> TCGLRKYKEPQLHSTGGLFTDITSHPWQAAIFAQNRRSSGERFLCGGILISSCWVLTAAHCFQESYLPDQLKVVLGRTYRVKPGEEEQTFKVKKYIVHKEFDDDTYNNDIALLQLKSDSPQCAQESDSVRAICLPEANLQLPDWTECELSGYGKHKSSSPFYSEQLKEGHVRLYPSSRCAPKFLFNKTVTNNMLCAGDTRSGEIYPNVHDACQGDSGGPLVCM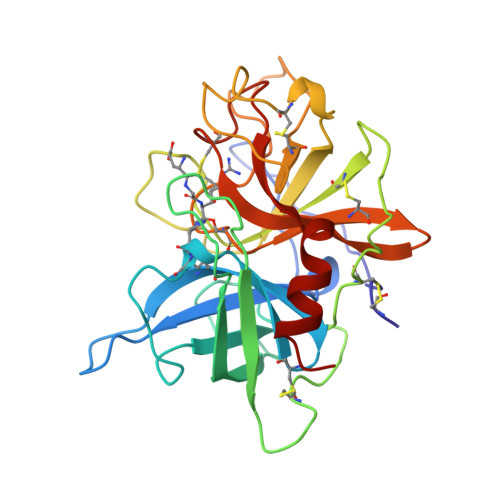NDNHMTLLGIISWGVGCGEKDVPGVYTKVTNYLGWIRDNMHL>GPPILKELENLSPEEAAHQKAVVETLLQEDPWRVAKMVKSYLQQHNIPQREVVDTTGLNQSHLSQHLNKGTPMKTQKRAALYTWYVRKQREVAQQFTHAGQGGLIEEPTGDELPTKKGRRNRFKWGPASQQILFQAYERQKNPSKEERETLVEECNRAECIQRGVSPSQAQGLGSNLVTEVRVYNWFANRRKEEAFRH[2x]

Hepatocyte nuclear factor 1A (HNF-1A) and HNF-4A are transcription factors that engage in crossregulatory gene transcription networks to maintain glucose-stimulated insulin secretion in pancreatic β cells. Variants in the HNF1A and HNF4A genes are associated with maturity-onset diabetes of the young (MODY). HNF-1A and HNF-4A form a crossregulatory loop, in which both factors regulate the respective other’s gene transcription. HNF-1A binds to the P2-HNF4A promoter and activates P2-driven gene transcription.

We therefore crystallized the protein-DNA complexes and determined their structures at 3.2 Å (P2 -169C>T) and 2.8 Å (P2 -181G>A, P2 -181G>T). A structural alignment of the 3 mutant complex structures and the DBD:P2 WT structure showed that there was no substantial change in overall conformation of the protein or the oligonucleotide. Interestingly, the mutation sites in all 3 P2 variants were in proximity to the same residues, which were Asn266 and Lys273 in helix α8. Lys273A in the P2 WT structure forms a hydrogen bond with the guanine base S.4G. Similar observations were made in the P2 -181G>T variant structure. The substitution of a guanine with a thymine (S.5G>T) leads to an introduction of a hydrophobic methyl group, likely leading to unfavorable interactions with Lys273A. The KD values of the P2 -181G>A and P2 -181G>T interaction were intermediate, with 0.6 μM and 0.7 μM, respectively. The strongest effects were observed for the P2 -181G>T variant, for which the kon rate was ~3 times lower and the koff rate ~3 times higher than for the P2 WT sequence. The resulting KD values from the kinetic analyses reflect the impaired HNF-1A binding, as the KD values were 5 (P2 -169C>T) to 10 (P2 -181G>T) times higher than for the P2 WT sample. For both expression plasmids, we observed a statistically significant decrease in normalized HNF-1A transcriptional activity for the 3 P2 variants within the HNF-1A binding site (P2 -169C>T, P2 -181G>A, P2 -181G>T) compared with the P2 WT reporter, which was in accordance with our in vitro data.> P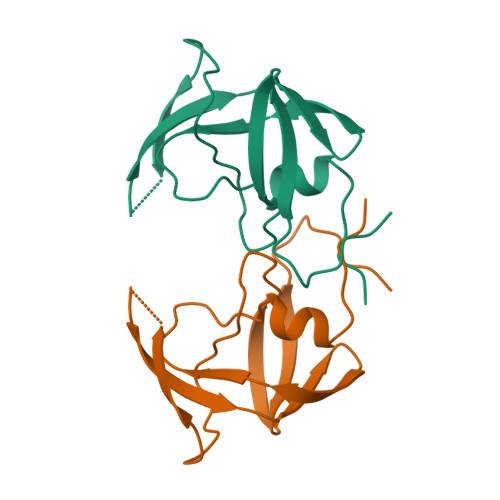QFHLWKRPVVTAHIEGQPVEVLLDTGADDSIVTGIELGPHYTPKIVGGIGGFINTKEYKNVEVEVLGKRIKGTIMTGDTPINIFGRNLLTALGMSLNF>MKTNKILAIGLLAAATVLTTGCSDSFLEVENPTGEPLEDYYTTDEHIQEALIAAYDPLHWPDWGLGQYNALNIDGEIMGDNFWVGGATKTDMQNWHMLFNYEANENNTLGSLWTVDYSGIKRCNDLLKYLDWGTDVTEANRKLYEMQARLLRVFYYNMLWHYFGNVPFYLENLSEPPYTAPQYTADQVYAELIAELEAVIDSKVLPLKYYKTIKEGKEVDDEGQLGRVTQAMAYMVYAEMVMYQNDESRFSKALGYMKELIDSPSFRLNPSFANIWETEGEWCDESIWEINYEQTNNERGWGSPLAVGGTVLPTLISPNSFPGDDGWSKGNDGWGFMPMRLETYQMFSEQDKRRDATCWVIAEDVEYTKRYQDTHIWLQKYRPYDKNFKQSSGD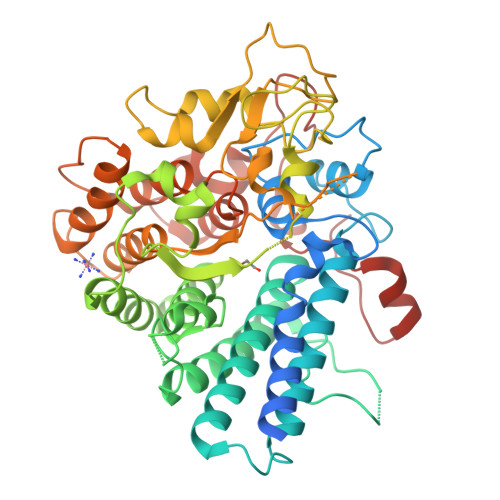QNLNYNNNYRYYRYAETLLNAAELSLRTGGSGTGEAKTWLNEVRTRAGLAGLANVTVDDVLTERRLEFVGEGKRYFDLVRAEGISGASASNKATTALVPDEYGYRTNSWTAKKKYIPIAQGELDSDPALVQNAYK[2x]> SSIEKNFIALENKNATVEQTKENIFLVPLKHLRDSQFVGELLVGTPPQTVYPIFDTGSTNVWVVTTACEEESCKKVRRYDPNKSKTFRRSFIEKNLHIVFGSGSISGSVGTDTFMLGKHLVRNQTFGLVESESNNNKNGGDNIFDYISFEGIVGLGFPGMLSAGNIPFFDNLLKQNPNVDPQFSFYISPYDGKSTLIIGGISKSFYEGDIYMLPVLKESYWEVKLDELYIGKERICCDEESYVIFDTGTSYNTMPSSQMKTFLNLIHSTACTEQNYKDILKSYPIIKYVFGELIIELHPEEYMILNDDVCMPAYMQIDVPSERNHA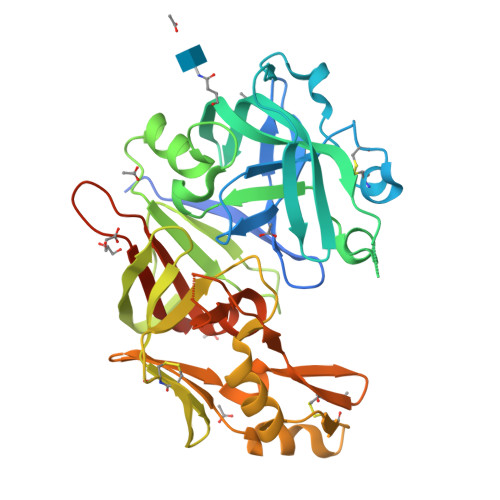YLLGSLSFMRNFFTVFVRGTESRPSMVGVARAKSKNENLYFQGHHHHHHHH> MTGPHAAGGSNHRTARLVAIIAGLLGTLMAIATPLLPVEQTTAELNWPQNGVWQSVDAPLIGYVATDLTVTVPCQAAAGLVGPENRNRSVLLSTVPKQAPKAIDRGLLIERINNDLTVIVRNTPVVSAPLEQVLSPDCRYLTFTAHADKVTGEFVGLTQGPDDDDPGEAVRGERSGYDFRPQIVGVFTDLSGPAPEGLQLSATIDTRYSTSPTLLKLLAMIVGVAMTVIALGALHVLDCADGRRHKRFLPSRWWSMTPLDGLVSAMLVWWHFVGANTADDGYILTMARVSEHAGYMANYYRWFGTPESPFGWYYDLLALWAHVSTASVWMRFPTLLMGLACWWVISREVIPRLGAAAKHSRAAAWTAAGLFLAFWLPLNNGLRPEPIIALGILLTWCSVERGVATSRLLPVAVAIIIGALTLFSGPTGIAAVGALLVAIGPLKTIVAAHVSRFGYWALLAPIAAAGTVTIFLIFRDQTLAAELQASSFKSAVGPSLAWFDEHIRYSRLFTTSPDGSVARRFAVLTLLLALAVSIAMTLRKGRIPGTALGPSRRIIGITIISFLAMMFTPTKWTHHFGVFAGLAGCLGALAAVAVTTTAMKSRRNRTVFGAAVLFVTALSFATVNGWWYVSNFGVPWSNSFP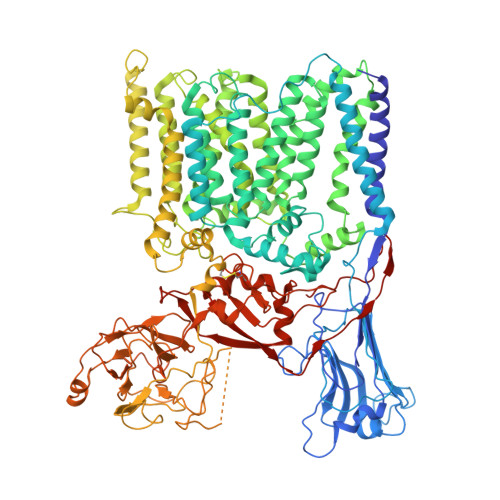EFKFGFTTMLLGLSVLALLVAAWFHFSGRDVSPDRPQRRWQRLLVAPLAVATWALVIFEVVSLTLGMINQYPAWSVGRSNLNALTGKTCGLANDVLVEQNANAGMLTPIGEPAGQALGAVTSLGFGPNGIPSDVSADPVMEQPGTDNFADSDSGVVTGTEVGTEGGTTAAAGINGSRARLPYGLNPATTPVLGSWRSGTQQPAVLRSAWYRLPDRDQAGPLLVVSAAGRFDQGEVEVQWATDEQAAANEPGGSITFGDVGAAPAWRNLRAPLSSIPPEATQIRLVASDDDLAPQHWIALTPPRIPELRTLQEVVGSSDPVMLDWLVGLAFPCQRPFDHRYGVVEVPKWRILPDRFGAEANSPVMDYLGGGPLGITELLLRPSSVPTYLKDDWYRDWGSLQRLTPWYPDAQPARLDLGTATRSGWWSPAPLRLSHHHHHHHHHH> MKASNYQEIAKAAILAGGLAAAGVLSVGESAQAQFIGTASQSRVSAAVTSI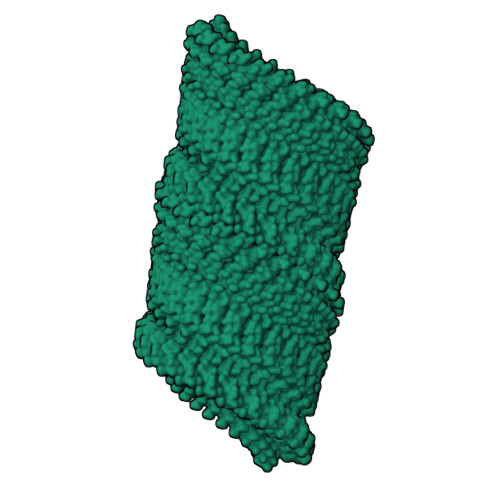LTDGNAAATNSFAVEQVLPSSDYVFSGVVAVQVSYATTISVGVGTAGALTPVITAAELTAPVVVNAGTQLTVERATADAISKAATGSRFGDVSGIVRAWSAGTSVLD>[2x]MKERFMSKFAIVFPG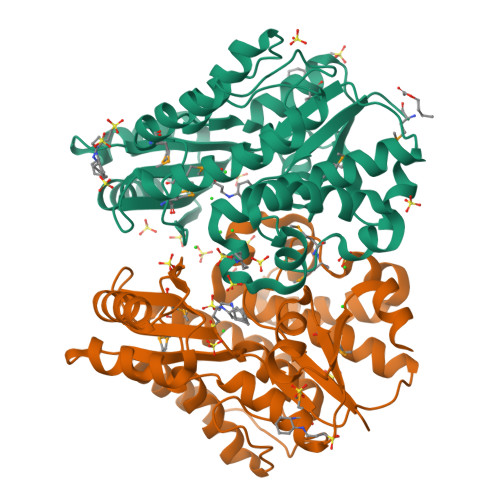QGSQAVGMLADLAEQYAVVKQTFAEASEVLGYDLWALVQDGPVEDLNQTFRTQPALLAASVAIWRVWQQLGLEQPAVLAGHSLGEYSALVCAGVIDFKQAIKLVELRGQLMQQAVPAGTGAMYAIIGLEDEAIAKACADAAQGEVVSPVNFNSPGQVVIAGQKDAVERAGVLCKEAGAKRALPLPVSVPSHCALMKPAADELAKTLAELEFNAPQIPVINNVDVVAETDPVKIKDALIRQLYSPVRWTECVEQMSAQGVEKLIEMGPGKVLTGLTKRIVKTLEGVAVNDVASLDAVK>MPKKPLIDQLHHEDSWRLFRILAEFVEGFETLSELQVPLVSVFGSARFGEGHPAYEAGYRLGRALAEAGFGVVTGGGPGVMEAVNRGAYEAGGVSVGLNIELPHEQKPNPYQTHALSLRYFFVRKVL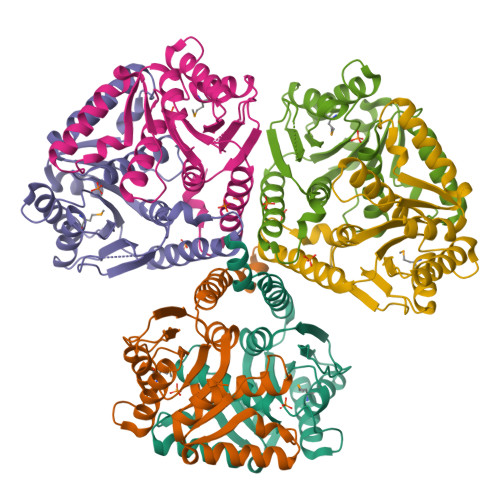FVRYAVGFVFLPGGFGTLDELSEVLVLLQTEKVHRFPVFLLDRGYWEGLVRWLAFLRDQKAVGPEDLQLFRLTDEPEEVVQALKAEAPPR[6x]>AAGEKT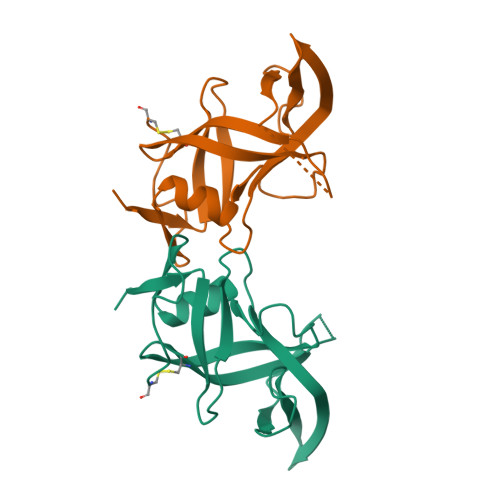VYGLNEYAALDGINLEVAAKLDTGAKTASLSARDIKRFKRNGESWVRFYLAIDAAHSHPIERPLARVSKIKRRAGDYDPEEGKKYTARPVIELDICMGSAMRSIEVNLTDRSAFQYPLLIGSEALKRFDALVDPSLKYAAGKPACAIAAHTAE[2x]> GSEESELYHAQIHLYKHVYNFVSSMALKSAMELGIADAIHNHGKPMTLSELASSLKLHPSKVNIL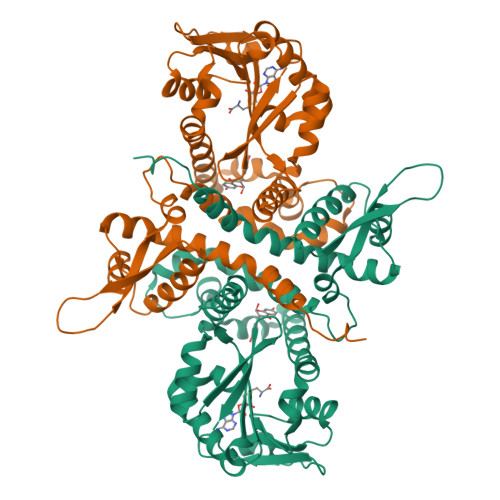HRFLRLLTHNGFFAKTIVKGKEGDEEEEIAYSLTPPSKLLISGKPTCLSSIVKGALHPSSLDMWSSSKKWFNEDKEQTLFECATGESFWDFLNKDSESSTLSMFQDAMASDSRMFKLVLQENKRVFEGLESLVDVGGGTGGVTKLIHEIFPHLKCTVFDQPQVVGNLTGNENLNFVGGDMFKSIPSADAVLLKWVLHDWNDEQSLKILKNSKEAISHKGKDGKVIIIDISIDETSDDRGLTELQLDYDLVMLTMFLGKERTKQEWEKLIYDAGFSSYKITPISGFKSLIEVYP>[2x]SKLVGGFSEWKDPDAYTTKIVKAMESKLFEKLSLPNQPEVSF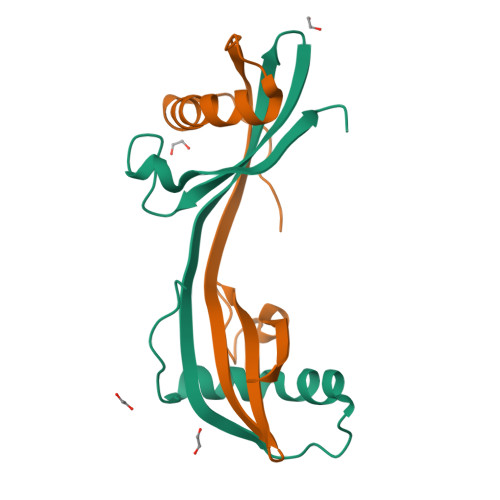LRYREQIVSGVNYCMRVKIGSDFYDLHIYVPLGSTGDIKSHLIQLTDLHLASELTHSH> MKIGSVIESSPHSILVKIDTLKIFEKAKSALQIGKYLKIQEGNHNFVLCVIQNIKISTDKDEDIFILTVQPVGIFKGEEFFQGNSMLPSPTEPVFLVEDDILNKIFSNEKTKIFHLGNLAQNEEVSFTLDGDKFFSKHVAVVGSTGSGKSCAVAKILQNVVGINDARNINKSDKKNSHIIIFDIHSEYKSAFEIDKNEDFNLNYLDVEKLKLPYWLMNSEELETLFIESNEQNSHNQVSQFKRAVVLNKEKYNPEFKKITYDSPVYFNINEVFNYIYNLNEEVINKIEGEPSLPKLSNGELVENRQIYFNEKLEFTSSNTSKATKASNGPFNG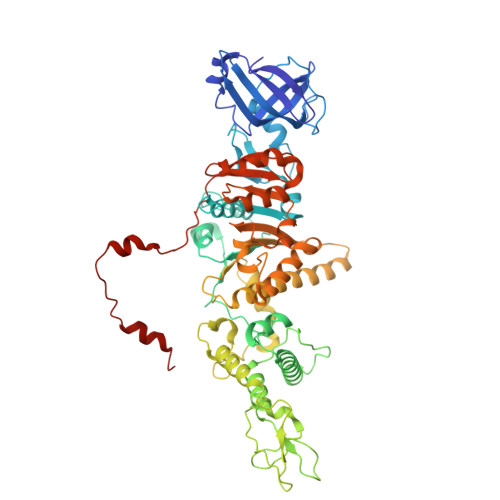EFNRFLSRFETKLTDKRLEFLLLNQDVEENSKYRTEHFEDILKQFMGYLDRSNVSIIDLSGIPFEVLSITISLISRLIFDFAFHYSKLQHQKDELNDIPFMIVCEEAHNYIPRTGGIEFKAAKKSIERIAKEGRKYGLSLMVVSQRPSEVSDTILSQCNNFINLRLTNINDQNYIKNLLPDNSRSISEILPTLGAGECLVVGDSTPIPSIVKLELPNPEPRSQSIKFHKKWSESWRTPSFEEVIMRWRKENG> MIPVLTSKKASELPVSEVASILQADLQNGLNKCEVSHRRAFHGWNEFDISEDEPLWKKYISQFKNPLIMLLLASAVISVLMHQFDDAVSITVAILIVVTVAFVQEYRSEKSLEELSKLVPPECHCVREGKLEHTLARDLVPGDTVCLSVGDRVPADLRLFEAVDLSIDESSLTGETTPCSKVTAPQPAATNGDLASRSNIAFMGTLVRCGKAKGVVIGTGENSEFGEVFKMMQAEEAPKTPLQKSMDLLGKQLSFYSFGIIGIIMLVGWLLGKDILEMFTISVSLAVAAIPEGLPIVVTVTLALGVMRMVKKRAIVKKLPIVETLGCCNVICSDKTGTLTKNEMTVTHIFTSDGLHAEVTGVGYNQFGEVIVDGDVVHGFYNPAVSRIVEAGCVCNDAVIRNNTLMGKPTEGALIALAMKMGLDGLQQDYIRKAEYPFSSEQKWMAVKCVHRTQQDRPEICFMKGAYEQVIKYCTTYQSKGQTLTLTQQQRDVYQQEKARMGSAGLRVLALASGPELGQLTFLGLVGIIDPPRTGVKEAVTTLIASGVSIKMITGDSQETAVAIASRLGLYSKTSQSVSGEEIDAMDVQQLSQIVPKVAVFYRASPRHKMKIIKSLQKNGSVVAMTGDGVNDAVALKAADIGVAMGQTGTDVCKEAADMILVDDDFQTIMSAIEEGKGIYNNIKNFVRFQLSTSIAALTLISLATLMNFPNPLNAMQILWINIIMDGPPAQSLGVEPVDKDVIRKPPRNWKDSILTKNLILKILVSSIIIVCGTLFVFWRELRDNVITPRDTTMTFTCFVFFDMFNALSSRSQTKSVFEIGLCSNRMFCYAVLGSIMGQLLVIYFPPLQKVFQTESLSILDLLFLLGLTSSVCIVAEIIKKVERSREKIQKHV

Secretory-pathway Ca2+-ATPases (SPCAs) play critical roles in maintaining Ca2+ homeostasis, but the exact mechanism of SPCAs-mediated Ca2+ transport remains unclear. Here, we determined six cryo-electron microscopy (cryo-EM) structures of human SPCA1 (hSPCA1) in a series of intermediate states, revealing a near-complete conformational cycle. The overall structure of hSPCA1 is typical of a P-type ATPase, with ten transmembrane (TM) helices (TM1–TM10) and three conserved cytosolic domains: the actuator (A), phosphorylation (P), and nucleotide-binding (N) domains. Structural analysis revealed that the Ca2+ coordinates with the side-chain oxygen atoms of several residues, including Glu308, Asn738, and Asp742, and the main-chain carbonyl oxygen atoms of other residues, including Val303, Ala304, and Ile306, consistent with the results reported by Chen et al. We also found that the Ca2+-binding site in hSPCA1 corresponds to site II in hSERCA2.

To gain insight into how hSPCA1 recognizes Ca2+, we successfully obtained the structures of hSPCA1 bound to Ca2+ in three different states: CaE1, CaE1-ATP, and CaE1P-ADP. These structures had resolutions of 3.59 Å, 3.52 Å, and 3.71 Å, respectively. We found that the TMDs were nearly identical in all three structures. The hydrolysis of ATP and transfer of a phosphate group to Asp350 in hSPCA1 resulted in the CaE1P-ADP state. The fact that the cytosolic headpiece remains open and that the TMD remains almost stationary in SPCAs during the phosphorylation reaction CaE1 → CaE1-ATP → CaE1P-ADP may represent a key feature that distinguishes them from other P-type II ATPases, such as SERCAs and NKAs. The N domain binds an ATP molecule and rotates ~57.0°, followed by ATP hydrolysis and phosphorylation of Asp350. This leads to the phosphorylated E1 state of hSPCA1 (the CaE1P-ADP state) with little changes in the overall structure.>[2x]NLNLPEQSTRFQTIASIHSNNCSFEILNNDPGYIYGDSVDGECRIAVAHRELGNGLERTGDDRFLFIFYALDNNNFIIANRHDGFVLQFLIANG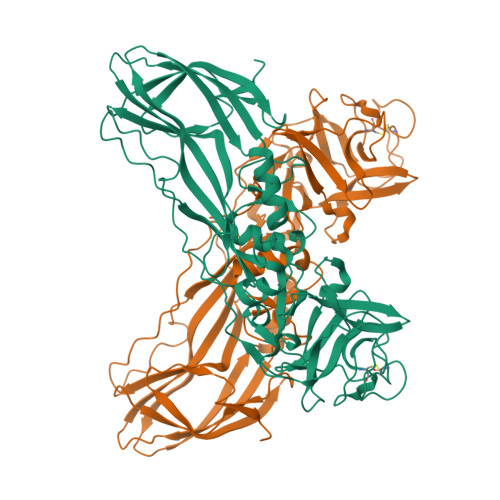QGVIVSREYQPNIHQEFTIQSINSDTFRLHSRDTNTFATVCWAQFNSWTKIVSRVDNPGAPNANLKHRSLLTDINMPQLPSLTPLQPLPRLTELEDGGLSPAQAPRAIIGRTLIPCLFVNDPVLRLENRIKQSPYYVLEHRQYWHRIWTDIFTAGERREYREVTGINNNAQNDMNKMINITIGADGPNRLRFGNLSTPFRQQIIDNSNTLGSFANTNYGTRTDIVNVFNSEFHQVRYARFVKAYEYRLTRADGSQVGTPWVVLDRKEMDLRTYPHNMAITLENVKIDNADNSYDLSIWKTPLKLKDGKIIIENHENSKPYYN>[2x]MNTVRSEKDSMGAIDVPADKLWGAQTQRSLEHFRISTEKMPTSLIHALALTKRAAAKVNEDLGLLSEEKASAIRQAADEVLAGQHDDEFPLAIWQTGSGTQSNMNMNEVLANRASELLGGVRGMERKVHPNDDVNKSQSSNDVFPTAMHV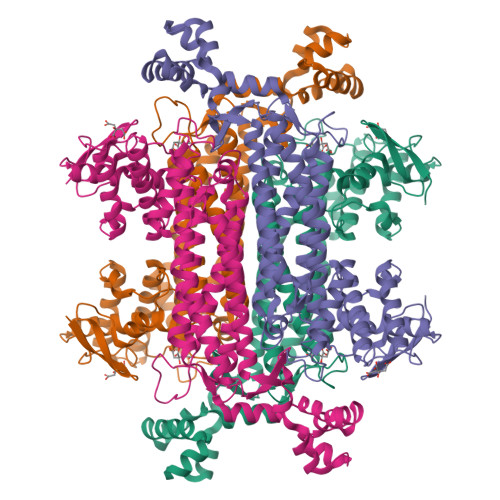AALLALRKQLIPQLKTLTQTLNEKSRAFADIVKIGRTHLQDATPLTLGQEISGWVAMLEHNLKHIEYSLPHVAELALGGTAVGTGLNTHPEYARRVADELAVITCAPFVTAPNKFEALATCDALVQAHGALKGLAASLMKIANDVRWLASGPRCGIGEISIPENEPGASIMPGKVNPTQCEALTMLCCQVMGNDVAINMGGASGNFELNVFRPMVIHNFLQSVRLLADGMESFNKHCAVGIEPNRERINQLLNESLMLVTALNTHIGYDKAAEIAKKAHKEGLTLKAAALALGYLSEAEFDSWVRPEQMVGSMKAGRHHHHH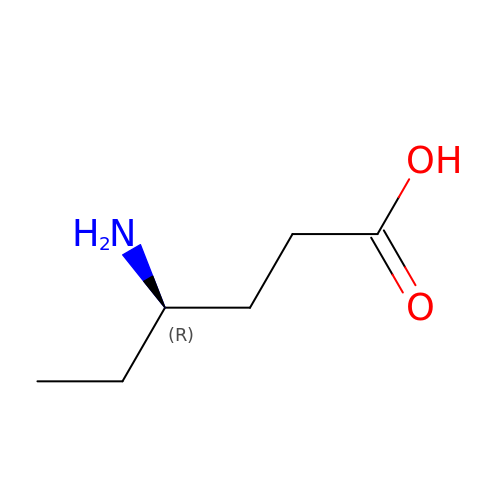4-AMINO HEXANOIC ACID | C6 H13 N O2 | ROFNJLCLYMMXCT-RXMQYKEDSA-N>[2x]MVPTR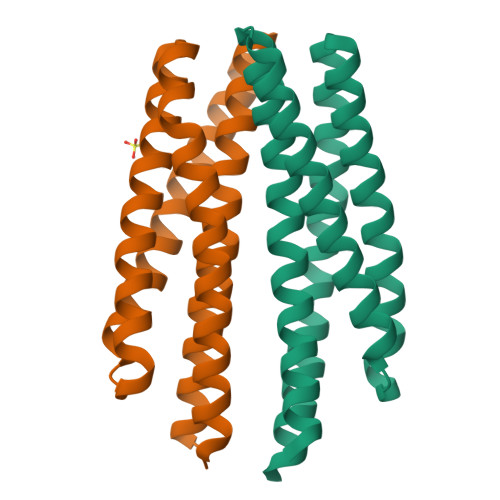STARMLANLKIRTGMFWVLSLFSLTLLFSTASAWWAALGSDQQITELDQTAHQSDRLNNALLMAIRSSANVSSGFIEQLGGHDESAGKRMALSVELNNKSQALVDEFVENAREPALRGLATELQATFAEYAKAVAGQREATRQRSLEQYFKVNSDAGNAMGRLQTLRQQLVTTLSERGQQIMLESDRRLARAQLLSLCLLGVTVVLAVLCWAFIAQRVLHPLREAGGHFRRIASGDLSVPVQGQGNNEIGQLFHELQRMQQSQRDTLGQINNCARQLDAAATALNAVTEESANNLRQQGQELEQAATAVTEMTTAVEEVARNAITTSQTTSESNQLAAQSRRQVSENIDGTEAMTREIQTSSAHLQQLVGQVRDIGKVLEVIRSVSEQTNLLALNAAIEAARAGEAGRGFAVVADEVRTLAYRTQQSTQEIEQMIGSVQAGTEAAVASMQASTNRAQSTLDVTLASGQVLEGIYSAIGEINERNLVIASAAEEQAQVAREVDRNLLNIRELSNHSAAGAQQTSEASKALSGLVGEMTALVGRFKV> GSPEFIEKNFVISDPRLPDNP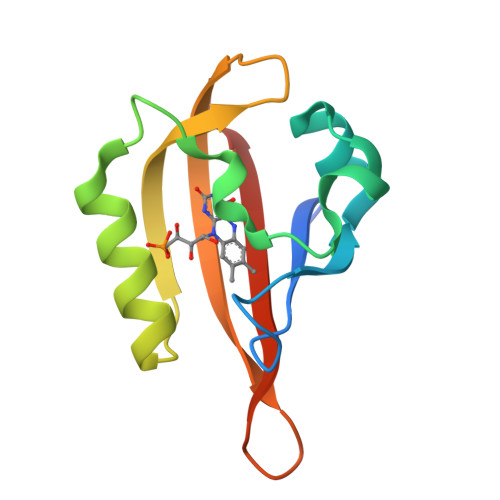IIFASDSFLELTEYSREEILGRNARFLQGPETDQATVQKIRDAIRDQREITVQLINYTKSGKKFWNLFHLQPMRDQKGELQYFIGVQLDGSDHV> GSHMERLCHPCPWEWTFFQGNCYFMSNSQRNWHDSITACKEVGAQLVVIKSAEEQNFLQLQSSRSNRFTWMGLSDLNQEGTWQWVDGSPLLPSFKQYWNRGEPNNVGEEDCAEFSGNGWNDDKCNLAKFWICKKSAASCSRDEEQFLSPAPATPNP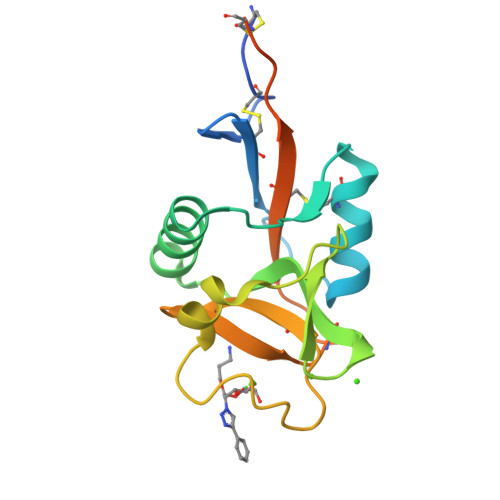PPA>SRKEIILTVWTNGNAIRKYTGQDKTISKYKLKDWY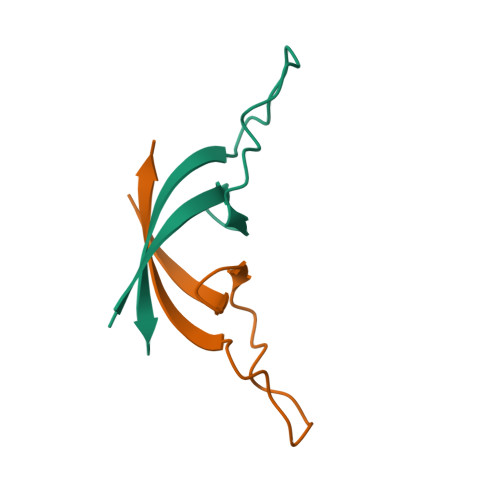KATAVITKEEETNETKTN[4x]> MSLSKKRKLESGDSGGAGAGGEGAEEENGGEQEAAPPRPRRTKSERDQLYYECYSDVSVHEEMIADQVRTEAYRLGILKNWAALRGKTVLDVGAGTGILSIFCAQAGARRVYAVEASAIWQQAREVVRLNGLEDRVHVLPGPVETVELPERVDAIVSEWMGYGLLHESMLSSVLHARTKWLKEGGLL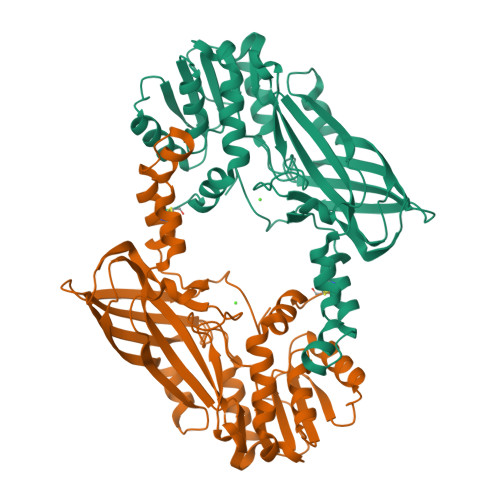LPASAELFVAPISDQMLEWRLGFWSQVKQHYGVDMSCMESFATRCLMGHSEIVVQDLSGEDVLARPQRFAQLELARAGLEQELEAGVGGRFRCSCYGSAPLHGFAVWFQVTFPGGDSEKPLVLSTSPLHPATHWKQALLYLNEPVPVEQDTDISGEITLLPSPDNPRRLRILLRYKVGDHEEKTKDFAMEDGSENLYFQ> GPMGKPARKGCEWKRFLKNNWVLLSTVAAVVLGITTGVLVREHSNLSTLEKFYFAFPGEILMRMLKLIILPLIISSMITGVAALDSNVSGKI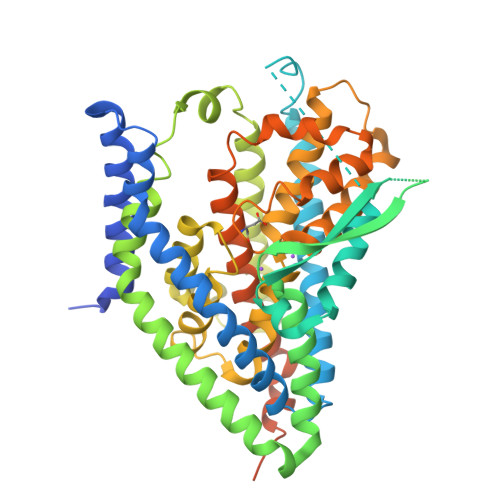GLRAVVYYFCTTLIAVILGIVLVVSIKPGVTQKVGEIARTGSTPEVSTVDAMLDLIRNMFPENLVQACFQQYKTKREEVKPPSDPEMTMTEESFTAVMTTAISKTKTKEYKIVGMYSDGINVLGLIVFCLVFGLVIGKMGEKGQILVDFFNALSDATMKIVQIIMCYMPLGILFLIAGKIIEVEDWEIFRKLGLYMATVLTGLAIHSIVILPLIYFIVVRKNPFRFAMGMAQALLTALMISSSSATLPVTFRCAEENNQVDKRITRFVLPVGATINMDGTALYEAVAAVFIAQLNDLDLGIGQIITISITATSASIGAAGVPQAGLVTMVIVLSAVGLPAEDVTLIIAVDWLLDRFRTMVNVLGDAFGTGIVEKLSKKELEQMDVSSEVNIVNPFALESTILDNEDSDTKKSYVNGGFAVDKSDTISFTQTSQF>ADVPAGVQLADKQTLVRNNGSEVQSLDPHKIEGVPESNVSRDLFEGLLISDVEGHPSPGVAEKWENKDFKVWTFHLRENAKWSDGTPVTAHDFVYSWQRLADPNTASPYASYLQYGHIANIDDIIAGKKPATDLGVKALDDHTFEVTLSEPVPYFYKLLVHPSVSPVPKSAVEKFGDKWTQPANIVTNGAYKLKNWVVNERIVLERNPQYWDNAKTVINQVTYLPISSEVTDVNRYRSGEIDMTYNNMPIELFQKLKKEIPNEVRVDPYLCTYYYEINNQKAPFNDVRVRTALKLALDRDIIVNKVKNQGDLPAYSYTPPYTDGAKLVEPEWFKWSQQKRNEEAKKLLAEAGFTADKPLTFDLLYNTSDLHKKLAIAVASIWKKNLGVNVNLENQEWKTFLDTRHQGTFDVARAGWCADYNEPTSFLNTMLSDSSNNTAHYKSPAFDKLIADTLKVADDTQRSELYAKAEQQLDKDSAIVPVYYYVNARLVKPWVGGYTGKDPLDNIYVKNLYIIKH[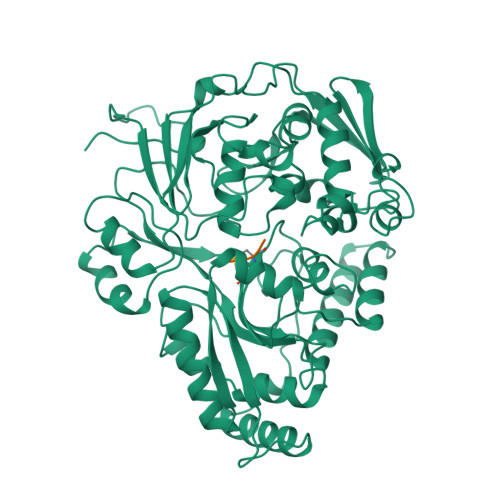2x];>KGK[2x]> GSDKERFARSDDEQSSADKERLARENHSEIERRRRNKMTAYITELSDMVPTCSALARKPDKLTILRMAVSHMKSLRGTGNTSTDGSYK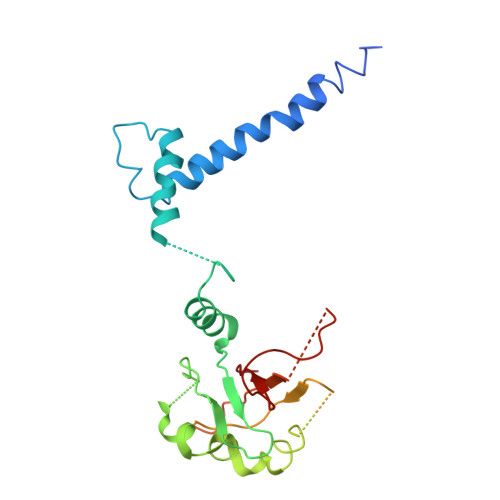PSFLTDQELKHLILEAADGFLFIVSCETGRVVYVSDSVTPVLNQPQSEWFGSTLYDQVHPDDVDKLREQLSTSENALTGRILDLKTGTVKKEGQQSSMRMCMGSRRSFICRMRCGSSSVDPVSVNRLSFVRNRCRNGLGSVKDGEPHFVVVHCTGYIKAWPPAGVSLPDDDPEAGQGSKFCLVAIGRLQVT>MPVNQSDNNQSEVVTRSATGIKNIVYIEVNDINPLNAGSYIMDDAPFFDYVILFAANIRGVGSDATLYNNPNVQYILDHKDTLIKPL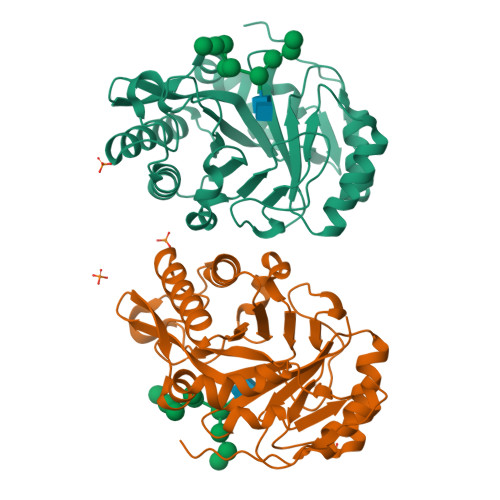QDKGIKVLLGLLGDHTGLGFANMNSAQTEQFATAVANAVSQYGLDGVDFADAWAEYGRNGYPSGSTGSFSNLITALHNKMPGKTITVFNYGYTSELTGVNSYIDYGIYAFFNSPSWSTGFGMPNSKFAPYTINLNSAPSAASAQLYSGQVASKGYGAIGYYDLRANNIVSVLNGVAKGAFKSTCTYDGNSYPKNY[2x]CCs are quaternary structures comprising two or more α-helices supercoiled around each other with cyclic (Cn) or dihedral (Dn) symmetry. Here, we describe variants with all combinations of the aliphatic residues, Ile, Leu and Val, at a and d to give four classes of peptide: the ββ class, with a and d = Ile or Val; Lβ, a = Leu and d = Ile or Val; βL, a = Ile or Val and d = Leu; and LL, a = d = Leu. Peptides are named systematically appending the one-letter code for the amino acids at the a and d sites to “CC-Type2-“; e.g., CC-Hept becomes CC-Type2-LI. In summary, solution-phase data and X-ray crystal structures demonstrate conclusively that different classes of Type-2 coiled-coil (CC) peptides—i.e., based on abcdefg repeats with predominantly hydrophobic residues at a, d, e and g—adopt a range of distinct states.

Finally, we tested the importance of β-branched residues at d in maintaining open-barrels outside of our designs. A recent design of a parallel pentameric α-helical barrel 5H2L_2.125 has a single Ile residue at d. We mutated this to Leu to give 5H2L_2.1-I9L. The peptide formed a stable 4-helix assembly in solution but crystallised as a mixed parallel/antiparallel CC pentamer, which is another low-symmetry structure. Thus, the single β-branched residues at d appears critical for specifying the open, all-parallel, α-helical barrel of 5H2L_2.125. In addition to a/d combinations, residues larger than Ala at the e and g sites influence the state adopted as they strongly specify against high-order blunt-ended barrels and fully collapsed states. This is demonstrated with the 5H2L_2.1-I9L mutant that lacks β-branched residues at the a and d positions. The sequence crystallises as an antiparallel pentameric barrel instead of forming a collapsed structure.

>XTQEYLLKELMKLLKEQIKLLKEQIKMLKELEKQX[5x]> VHFHPFGNVNFYEMDWSLKGDLWAHDPVIAKEGSRWYVFHTGSGIQIKTSEDGVHWENMGRVFPSLPDWCKQYVPEKDEDHLWAPDICFYNGIYYLYYSVSTFG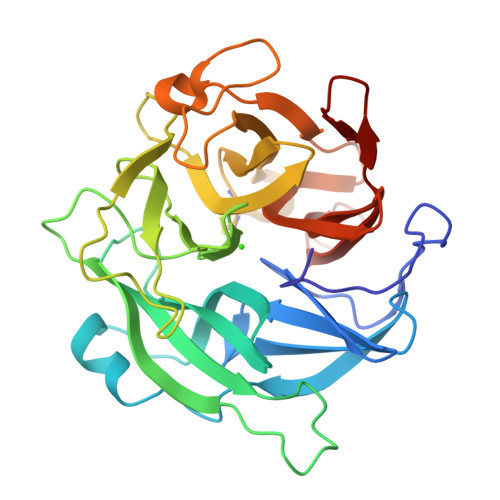KNTSVIGLATNRTLDPRDPDYEWKDMGPVIHSTASDNYNAIDPNVVFDQEGQPWLSFGSFWSGIQLIQLDTETMKPAAQAELLTIASRGEEPNAIEAPFIVCRNGYYYLFVSFDFCCRGIESTYKIAVGRSKDITGPYVDKNGVSMMQGGGTILDAGNDRWIGPGHCAVYFSGVSAILVNHAYDALKNGEPTLQIRPLYWDDEGWPYL>[3x]MKSPIPLRDVPQSNIFRKGDVFVLFGELFGRGYANGLINEARDAGMTIVGITVGRRDENNALRALTAEELATAEANLGGRIINVPLMAGFDLDAPAGEPTPTDLLADMTLKSWQDDKLDWAHIEKCRAVGVQRFKDGVAKVMAELDGMIPDGANAFFAHTMAGGIPKVKVFLAIANRIYKGRGERFL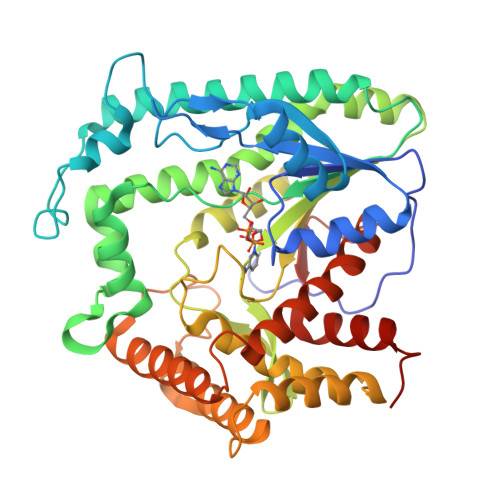SSSALLNSDLGKLILMNFDEVTANTFLHLIEGSAAIRARLEKSGGQVRYSAYGYHGTEILIDDKYQWQTYTSYTQGKAKMRLERIAEDAWKQGIKATVYNCPEIRTNSSDIFVGVELSLFPLLKALKKENGGAWAEAQWQACREVLSEGHTLESLLQKIDDYNASDVMKGFRNFEAWPMPNTAELADIMIGTSDEITKMHKSRDALVTDVLSALVLEGTGPLMFHESSNPAGPVLWLSHDVIAKQLNLMHRLEHHHHHH> MTFRKSFDCYDFYDRAKVGEKCTQDDWDLMKIPMKAMELKQKYGLDFKGEFIPTDKDMMEKLFKAGFEMLLECGIYCTDTHRIVKYTEDEIWDAINNVQKEFVLGTGRDAVNVRKRSVGDKAKPIVQGGPTGSPISEDVFMPVHMSYALEKEVDTIVNGVMTSVRGKSPIPKSPYEVLAAKTETRLIKNACAMAGRPGMGVKGPETSLSAQGNISADCTGGMTCTDSHEVSQLNELKIDLDAISVIAHYKGNSDIIMDEQMPIFGGYAGGIEETTIVDVATHINAVLMSSASWHLDGPVHIRWGSTNTRETLMIAGWACATISEFTDILSGNQYYPCAGPCTEMCLLEASAQSITD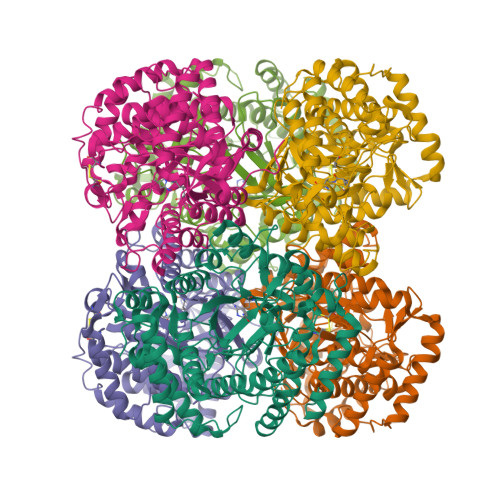TASGREILSGVASAKGVVTDKTTGMEARMMGEVARATAGVEISEVNVILDKLVSLYEKNYASAPAGKTFQECYDVKTVTPTEEYMQVYDGARKKLEDLGLVF>[2x]MLVKGNEILLKAHKEGYGVGAFNFVNFEMLNAIFEAGNEENSPLFIQASEGAIKYMGIDMAVGMVKIMCERYPHIPVALHLDHGTTFESCEKAVKAGFTSVMIDASHHAFEENLELTSKVVKMAHNAGVSVEAELGRLMGIEDNISVDEKDAVLVNPKEAEQFVKESQVDYLAPAIGTSHGAFKFKGEPKLDFERLQEVKRLTNIPLVLHGASAIPDNVRKSYLDAGGDLKGSKGVPFEFL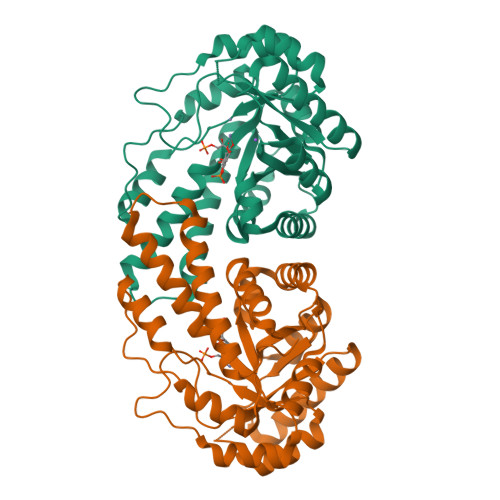QESVKGGINKVNTDTDLRIAFIAEVRKVANEDKSQFDLRKFFSPAQLALKNVVKERMKLLGSANKI> SEISRQEFQRRRQALVEQMQPGSAALIFAAPEVTRSADSEYPYRQNSDFWYFTGFNEPEAVLVLIKSDDTHNHSVLFNRVRDLTAEIWFGRRLGQDAAPEKLGVDRALAFSEINQQLYQLLNGLDVVYHAQGEYAYADVIVNSALEKLRKGSRQNLTAPATMIDWRPVVHEMRLFKSPEEIAVLRRAGEITAMAHTRAMEKCRPGMFEYHLEGEIHHEF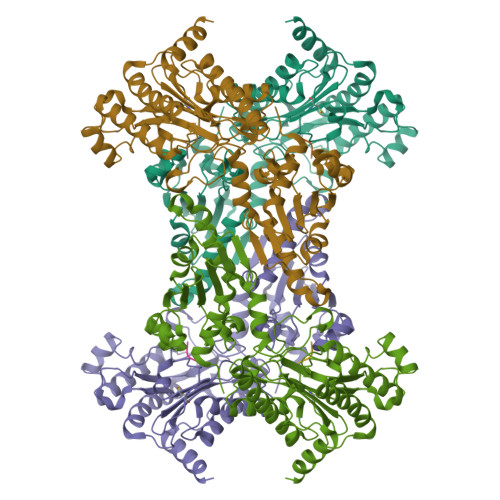NRHGARYPSYNTIVGSGENGCILAYTENECEMRDGDLVLIDAGCEYKGYAGDITRTFPVNGKFTQAQREIYDIVLESLETSLRLYRPGTSILEVTGEVVRIMVSGLVKLGILKGDVDELIAQNAHRPFFMHGLSHWLGLDVHDVGVYGQDRSRILEPGMVLTVEPGLYIAPDAEVPEQYRGIGIRIEDDIVITETGNENLTASVVKKPEEIEALMVAARKQ;> VPL>MTHDVPVTIDWPALRTQARDAMSRAYAPYSGYPVGAAALVDDGRTVTGCNVENASYGLGLCAEC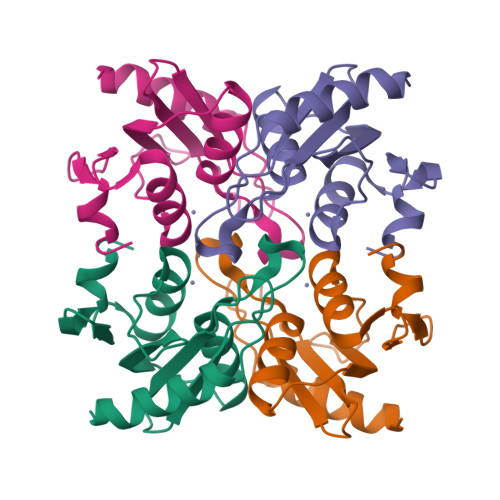GLVSALFASGGGRLTAFTCVDGKGELLVPCGRCRQLLHEHGGPDLLVDTAAGIRPLAALLPDAFGPGHLTR[2x]>[2x]GFKQDIATIRGDLRTYAQDIFLAFLNKYPDERRYFKNYVGKSDQELKSMAKFGDHTEKVFNLMMEVADRATDCVPLASDANTLVQDKQHSSLTTGNFEK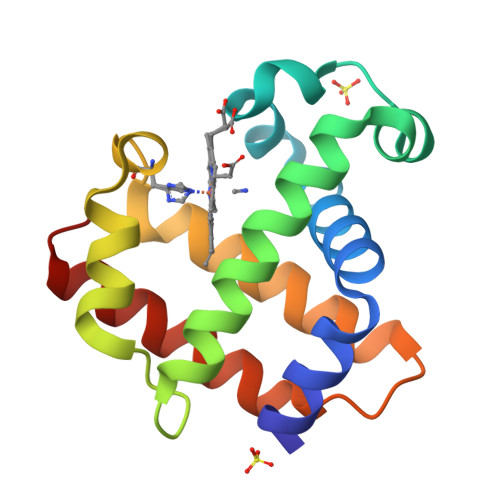LFVALVEYMRASGQSFDSQSWDRFGKNLVSALSSAGMK>[2x]MSTTNHDHHIYVLMGVSGSGKSAVASEVAHQLHAAFLDGDFLHPRR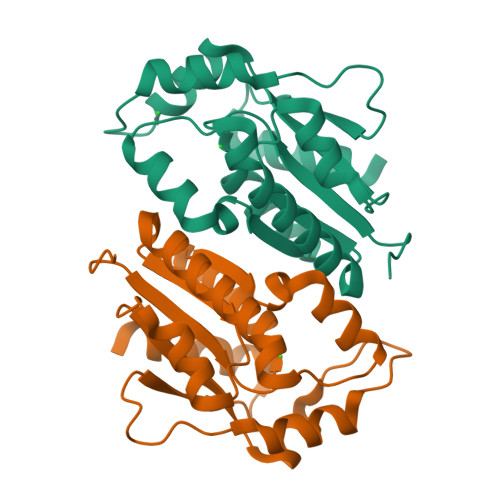NIEKMASGEPLNDDDRKPWLQALNDAAFAMQRTNKVSLIVCSALKKHYRDLLREGNPNLSFIYLKGDFDVIESRLKARKGHFFKTQMLVTQFETLQEPGADETDVLVVDIDQPLEGVVASTIEVIKKGK>[2x]SGISLDNSYKMDYPEMGLCIIINNKNFHKSTGMTSRSGTDVDAANLRETFRNLKYEVRNKNDLTREEIVELMRDVSKEDHSKRSSFVCVLLSHGEEGIIFGTNGPVDLKKITNFFRGDRCRSLTGKPKLFIIQACRGTELDCGIETDSGVDDDMACHKIPVEADFLYAYSTAPGYYSWRNSKDGSWFIQSLCAMLKQY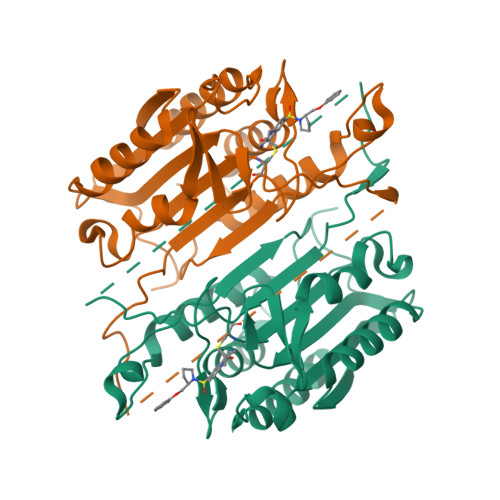ADKLEFMHILTRVNRKVATEFESFSFDATFHAKKQIPCIVSMLTKELYFYHHHHHHH Wall teichoic acid (WTA) is a polyol phosphate polymer that covalently decorates peptidoglycan of gram-positive bacteria, including Staphylococcus aureus. Central to WTA biosynthesis is flipping of lipid-linked precursors across the cell membrane by TarGH, a type V ABC transporter. TarGH is a heterotetramer composed of two TarG polytopic transmembrane domains (TMD) and two TarH nucleotide binding domains (NBD). Like other ABC transporters, TarGH uses the energy derived from the ATP hydrolysis cycle in the NBDs to drive substrate transport across the membrane via the TMDs.

To investigate if these differences were a result of targocil-II binding or the choice of ATP analogue, we determined structures of TarGH produced in L. lactis in complex with ATPγS alone and with targocil-II. In the presence of ATPγS and targocil-II, which is bound near identically to the AMP-PNP structure as above, we observe two approximately equally populated states of D-loopON (3.0 Å resolution) and D-loopOFF (2.7 Å resolution). However, the mixed population also suggests that D-loopON is less energetically favourable in the presence of ATPγS compared to AMP-PNP, where we only observe D-loopON, possibly due to steric or charge differences of the thiophosphate that could repel the approach of Val173. This hypothesis is also supported by the observed weaker binding of targocil-II in the presence of ATPγS.

>[2x]MGSSHHHHHHHHHHSSGLVPRGSHMSAIGTVFKEHVKNFYLIQRLAQFQVKIINHSNYLGVAWELINPVMQIMVYWMVFGLGIRSNAPIHGVPFVYWLLVGISMWFFINQGILEGTKAITQKFNQVSKMNFPLSIIPTYIVTSRFYGHLGLLLLVIIACMFTGIYPSIHIIQLLIYVPFCFFLTASVTLLTSTLGVLVRDTQMLMQAILRILFYFSPILWLPKNHGISGLIHEMMKYNPVYFIAESYRAAILYHEWYFMDHWKLMLYNFGIVAIFFAIGAYLHMKYRDQFADFL;>[2x]MNVSVNIKNVTKEYRIYRTNKERMKDALIPKHKNKTFFALDDISLKAYEGDVIGLVGINGSGKSTLSNIIGGSLSPTVGKVDRNGEVSVIAISAGLSGQLTGIENIEFKMLCMGFKRKEIKAMTPKIIEFSELGEFIYQPVKKYSSGMRAKLGFSINITVNPDILVIDEALSVGDQTFAQKCLDKIYEFKEQNKTIFFVSHNLGQVRQFCTKIAWIEGGKLKDYGELDDVLPKYEAFLNDFKKKSKAEQKEFRNKLDESRFVIK>[2x]GSNVADGLAWSYYFGYLKFVLPELEKQIEKTSKFRSKEKFVKKMFILIPSNCFWDDKIPGSDYDPQNRITFEGNTEPLEKTRGGVFL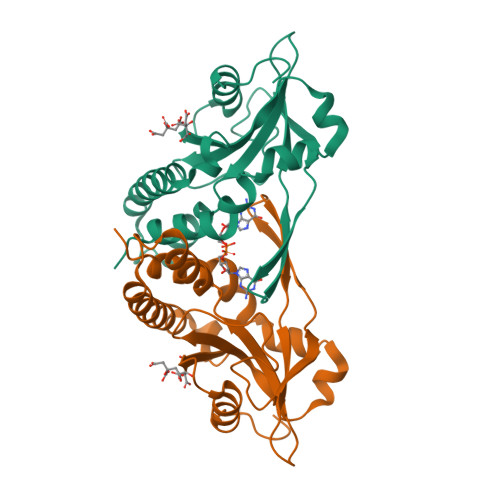RHYKHSVYEIKDGENEPWFCIMEYATPLLTLYDMSVAQPGELSREERDAQVVVFLRKLQDILEGDRACQGKYELVTFSPDRDLADVMLRKLKDSELEIGG>MATQAKRPRVAGPVDGGDLDPVACFLSWCRRVGLELSPKVAVSRQGTVAGYGMVARESVQAGELLFVVPRAALLSQHTCSIGGLLERERVALQSQSGWVPLLLALLHELQAPASRWRPYFALWPELGRLEHPMFWPEEERRCLLQGTGVPEAVEKDLANIRSEYQSIVLPFMEAHPDLFSLRVRSLELYHQLVALVMAYSFQEPLEEEEDEKEPNSPVMVPAADILNHLANHNANLEYSANCLRMVATQPIPKGHEIFNTYGQMANWQLIHMYGFVEPYPDNTDD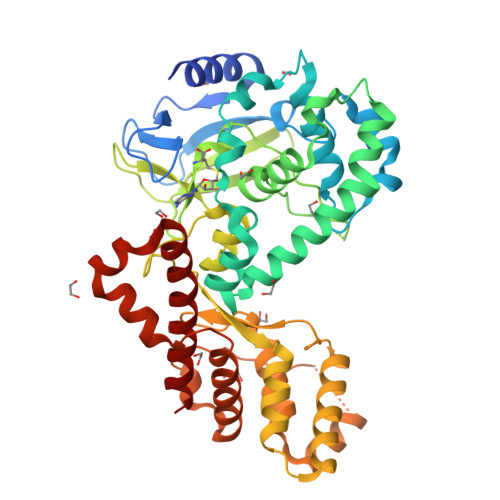TADIQMVTVREAALQGTKTEAERHLVYERWDFLCKLEMVGEEGAFVIGREEVLTEEELTTTLKVLCMPAEEFRELKDQDGGGDDKREEGSLTITNIPKLKASWRQLLQNSVLLTLQTYATDLKTDQGLLSNKEVYAKLSWREQQALQVRYGQKMILHQLLELTS[2x];>RKRTYETFKSIMKKS[2x]> MASYNFSLGEFSKTFKDYGTGSGKDVIADEKPFSILLMGVDTGSSERTSKWEGNSDSMILVTVNPKTKKTTMTSLERDILVKLSGSKTNDQTGYDAKLNAAYAAGGAKMAIMTVQDMLDIKIDKYVQINMEGLVQLVDAVGGITVTNHFDFPISIEEHEPEFTASVEPGTHKINGEQALVYSRMRYDDPDGDYGRQKRQREVISKVLKKILALDSVSKYRKILSAVSKNMQTNIEISSSTIPKLLGYSDALKSIRTYQLKGEGTTIDGGSYQLVTSKELLKAQNRIKGQLGLKKSTAENLKTTASLYENFY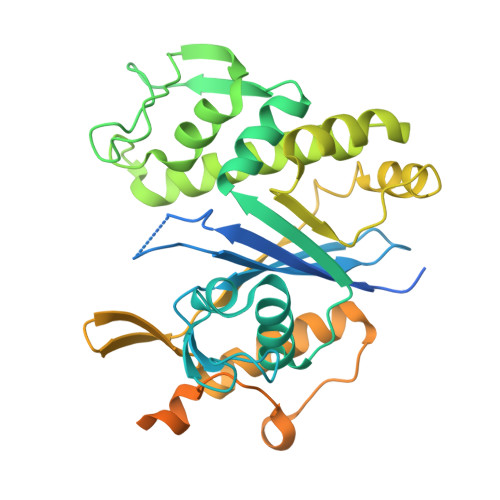GGDTSIYDSSSSASDYSSSGNYSGSSSDYGSSSSYGSNSSSGSSSDYSGQNSYNQGNYQQPAAGTGIGNLEHHHHHH> MQSVGGDSSADRLFPPQWICCDIRYLDVSILGKFAVVMADPPWDIHMELPYGTLTDDEMRRLNIPVLQDDGFLFLWVTGRAMELGRECLNLWGYERVDEIIWVKTNQLQRIIRTGRTGHWLNHGKEHCLVGVKGNPQGFNQGLDCDVIVAEVRST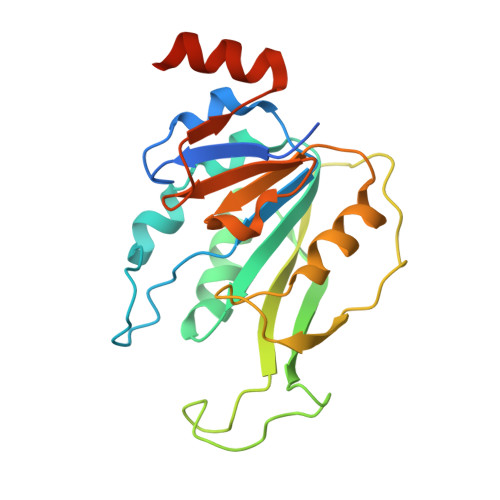SHKPDEIYGMIERLSPGTRKIELFGRPHNVQPNWITLGNQLDGIHLLDPDVVARFKQRYPDGIISKPKNL>MHHHHHHSNLLTVHQNLPALPVDATSDEVRKNLMDMFRDRQAFSEHTWKMLLSVCRSWAAWCKLNNRKWFPAEPEDVRDYLLYLQARGLAVKTIQQHLGQLNMLHRRSGLPRPSDSNAVSLVMRRIRKENVDAGERAKQALAFERTDFDQVRSLMENSDRCQDIRNLAFLGIAYNTLLRLAEIARIRVKDISRTDGGRMLIHIGRTKTLVSTAGVEKALSLGVTKLVERWISVSGVADDPNNYLFCRVRKNGVAAPSATSQ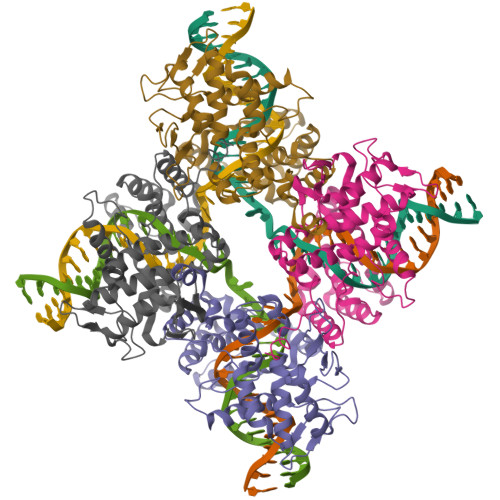LSNSALGGIFGATHRLIYGAKDDSGQRYLAWSGHSARVGAARDMARAGVSIPEIMQAGGWTNVNIVMNYIRNLDSETGAMVRLLEDGD[2x]>MKLVMAIIKPFKLDEVREALTSLGIQGLTVSEVKGFGRQKGQTEIYRGAEYSVSFLPKVKVEVAVSDDQYEQVVEAIQKAANTGRIGDGKIFVLDIAQAVR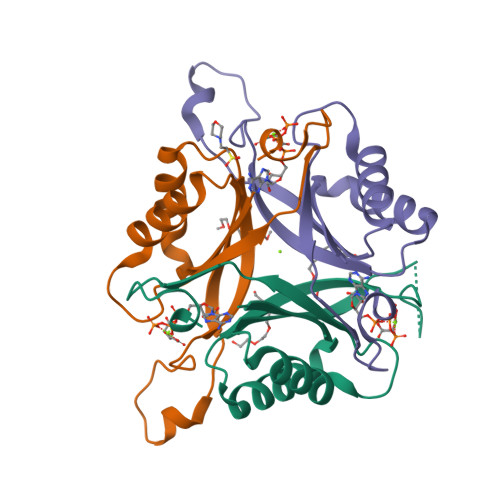IRTGETNTEAL[3x]N,N'-bis[3-(1,4,5,6-tetrahydropyrimidin-2-yl)phenyl]biphenyl-4,4'-dicarboxamide 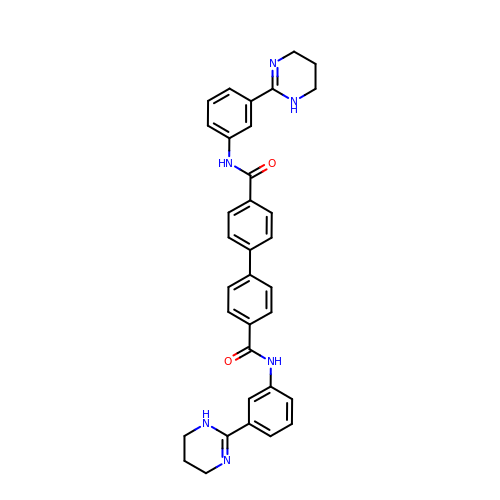| C34 H32 N6 O2 | FIDDBSXGDWEBNT-UHFFFAOYSA-N>TAPSQVLKIRRPDDWHLHLRDGDMLKTVVPYTSEIYGRAIVMPNLAPPVTTVEAAVAYRQRILDAVPAGHDFTPLMTCYLTDSLDPNELERGFNEGVFTAAKLYPANATTNSSHGVTSVDAIMPVLERMEKIGMPLLVHGEVTHADIDIFDREARFIESVMEPLRQRLTALKVVFEHITTKDAADYVRDGNERLAATITPQHLMFNRNHMLVGGVRPHLYCLPILKRNIHQQALRELVASGFNRVFLGTDSAPHARARKESSCGCAGCFNAPTALGSYATVFEEMNALQHFEAFCSVNGPQFYGLPVNDTFIELVREEQQVAESIALTDDTLVPFLAGETVRWSVKQ[2x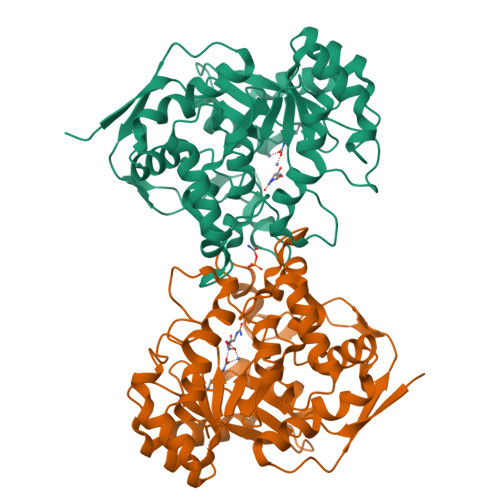]> HHHHHHGSMAKKPTALIILDGFANRESEHGNAVKLANKPNFDRYYNKYPTTQIEASGLDVGLPEGQMGNSEVGHMNIGAGRIVYQSLTRINKSIEDGDFFENDVLNNAIAHVNSHDSALHIFGLLSDGGVHSHYKHLFALLELAKKQGVEKVYVHAFLDGRDVDQKSALKYIEETEAKFNELGIGQFASVSGRYYAMDRDKRWERE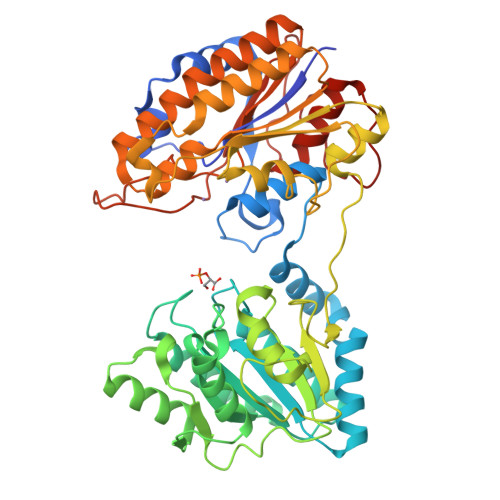EKAYNAIRNFDAPTYATAKEGVEASYNEGLTDEFVVPFIVENQNDGVNDGDAVIFYNFRPDRAAQLSEIFANRAFEGFKVEQVKDLFYATFTKYNDNIDAAIVFEKVDLNNTIGEIAQNNNLTQLRIAETEKYPHVTYFMSGGRNEEFKGERRRLIDSPKVATYDLKPEMSAYEVKDALLEELNKGDLDLIILNFANPDMVGHSGMLEPTIKAIEAVDECLGEVVDKILDMDGYAIITADHGNSDQVLTDDDQPMTTHTTNPVPVIVTKEGVTLRETGRLGDLAPTLLDLLNVEQPEDMTGESLIKH>[2x]MLGLKTSIIGRRVIYFQEITSTNEFAKT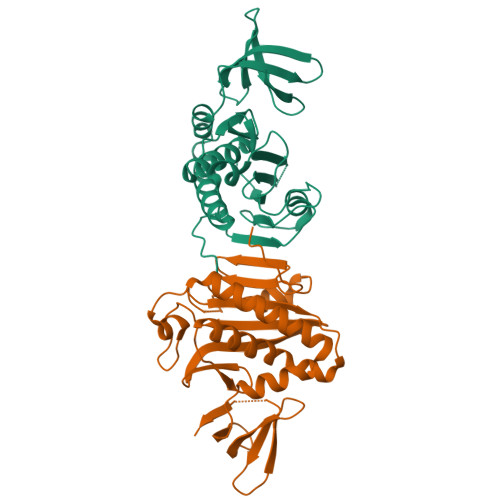SYLEEGTVIVADKQTMGHGRLNAKWESPEGGLWLSIVLSPKVPQKDLPKIVFLGAVGVVETLKEFSIDGRIKWPNDVLVNYKKIAGVLVEGKGDKIVLGIGLNVNNKVPNGATSMKLELGSEVPLLSVFRSLITNLDRLYLNFLKNPMDILNLVRDNMILGVRVKILGDGSFEGIAEDIDDFGRLIIRLDSGEVKKVIYGDVSLRFL> GSGAPPTDLQKMVMGNTKPVELILDGKTVAICCATGVFGTAYLVPRHLFAEKYDKIMLDGRAMTDSD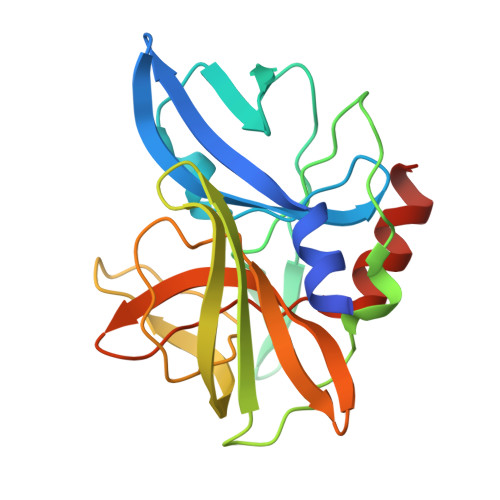YRVFEFEIKVKGQDMLSDAALMVLHRGNKVRDITKHFRDTARMKKGTPVVGVVNNADVGRLIFSGEALTYKDIVVLMDGDTMPGLFAYKAATRAGYAGGAVLAKDGADTFIVGTHSAGGNGVGYCSCVSRSMLQKMKAHVDPEPHHE> MSQQGLERRLLAGLQGLGLTINQAQRAVKHFGADALDRLEKDLFTLTEVEGIGFLTADKLWQARGGALDDP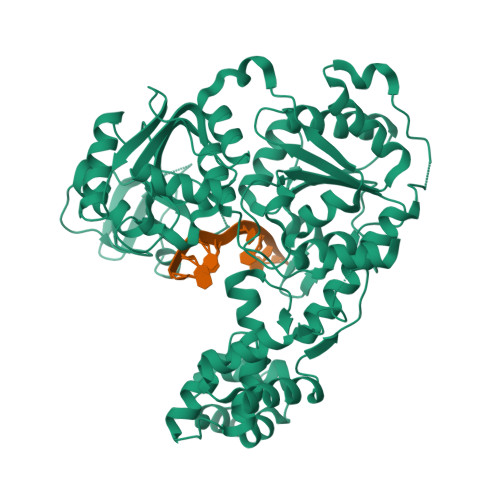RRLTAAAVYALQLAGTQAGHSFLPRSRAEKGVVHYTRVTPGQARLAVETAVELGRLSEDDSPLFAAEAAATGEGRIYLPHVLRAEKKLASLIRTLLATPPADGAGNDDWAVPKKARKGLSEEQASVLDQLAGHRLVVLTGGPGTGKSTTTKAVADLAESLGLEVGLCAPTGKAARRLGEVTGRTASTVHRLLGYGPQGFRHNHLEPAPYDLLIVDEVSMMGDALMLSLLAAVPPGARVLLVGDTDQLPPVDAGLPLLALAQAAPTIKLTQVYRQAAKNPIIQAAHGLLHGEAPAWGDKRLNLTEIEPDGGARRVALMVRELGGPGAVQVLTPMRKGPLGMDHLNYHLQALFNPGEGGVRIAEGEARPGDTVVQTKNDYNNEIFNGTLGMVLKAEGARLTVDFDGNVVELTGAELFNLQLGYALTVHRAQGSEWGTVLGVLHEAHMPMLSRNLVYTALTRARDRFFSAGSASAWQIAAARQREARNTALLERIRAHLEHHHHHH>ATSMDVFVLDTSVF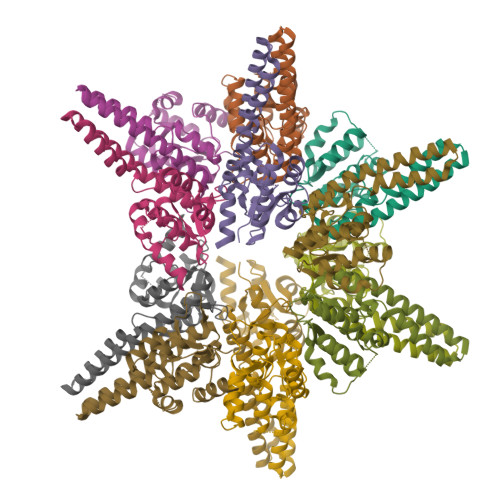TNPEIYRTFEEDQRGAMETFIHLALNSRAEFYMPTSVYTEMRKIMDVGELWAEFEMVVKIRSPRRFQLTVPADFLYEFIEELRYRINKGLRIAEEHTREASGCEDVGKLIARLREKYREALRQGILDSKEDVDVLLLAYELDGVLVSADEGLRTWADKIGIKLIDPKNFKNILESLVRHRF[12x]> 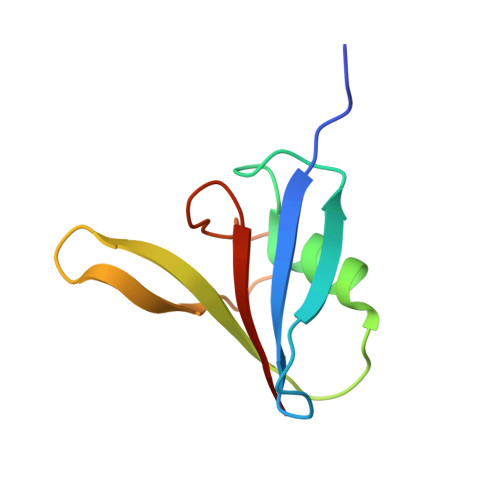GPAAASTKVLYYTDRSLTPFLVNIPKRLGDVTLQDFKAAVDRHGSFRYHFKSLDPEFGTVKEEVFQDDAVIPGWEGKIVAWVEED>AIAAQKISEAHEHIAKAEKYLKTSF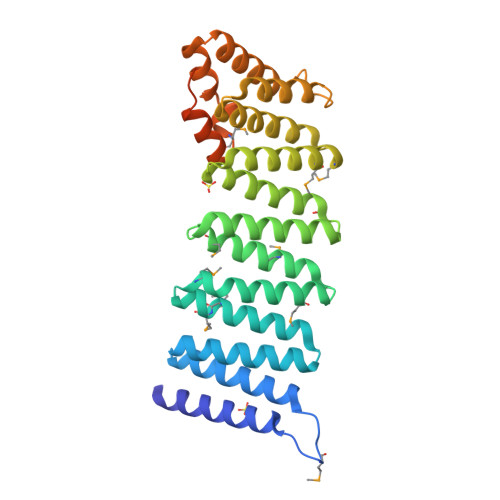MKWKPDYDSAASEYAKAAVAFKNAKQLEQAKDAYLQEAEAHANNRSLFHAAKAFEQAGMMLKDLQRMPEAVQYIEKASVMYVENGTPDTAAMALDRAGKLMEPLDLSKAVHLYQQAAAVFENEERLRQAAELIGKASRLLVRQQKFDEAAASLQKEKSMYKEMENYPTCYKKCIAQVLVQLHRADYVAAQKCVRESYSIPGFSGSEDCAALEDLLQAYDEQDEEQLLRVCRSPLVTYMDNDYAKLAISLKVPGGGGGKKKPSASASAQPQEEEDDEYAGGLC[4x]> MDPQGDAAQKTDTSHHDQDHPTFNKITPNLAEFAFSLYRQLAHQSNSTNILFSPVSIAAAFAMLSLGAKGDTHDEILEGLNFNLTEIPEAQIHEGFQELLRTLNQPDSQLQLTTGNGLFLSEGLKLVDKFLEDVKKLYHSEAFTVNFGDTEEAKKQINDYVEKGTQGKIVDLVKELDRDTVFALVNYIFFKGKWERPFEVKDTEEEDFHVDQVTTVKVPMMKRLGMFNIQHSKKLSSWVLLMKYLGNATAIFFLPDEGKLQHLENELTHDIITKFLENEDRRSASLHL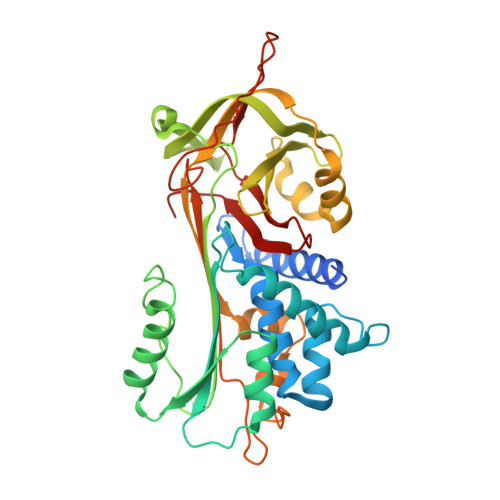PKLSITGTYDLKSVLGQLGITKVFSNGADLSGVTEEAPLKLSKAVHKAVLTIDEKGTEAAGAMFLEAIPRSIPPEVKFNKPFVFLIIEQNTKAPLFMGRVVNPTQK> SLSGMELSYRRSDLIFKRPAGTSRGVLTSKPTWFVRLDIDGHGGQGEVSLIPGLSLDPEEQIGRELDLLARRLRAEEPIRLRQFLAERGGADFSDYRSVLTDIAGILDSWQVSTDGRFPALRFALEMALLDLLSGGRQEWFASDFTRGEKRIPVNGLIWMGEAAFMQEQIEAKLAEGYGCLKLKIGAIDFDKE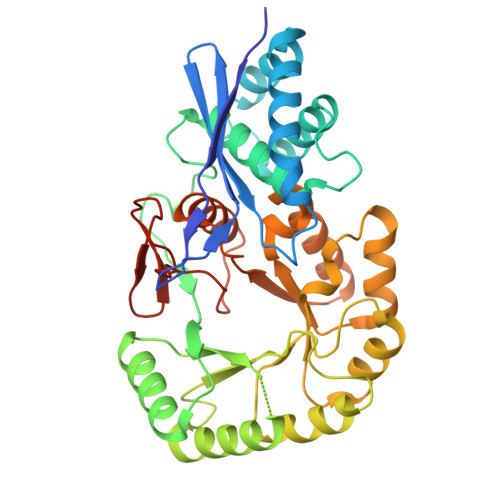CALLAGIRESFSPQQLEIRVDANGAFSPANAPQRLKRLSQFHLHSIEQPIRQHQWSEMAALCANSPLAIALDEELIGLGAEQRSAMLDAIRPQYIILKPSLLGGFHYAGQWIELARERGIGFWITSALESNLGLAAIAQWTALYQPTMPQGLGTGQLYTNNLPSNLAVDGGLLGVSEGHHHHHH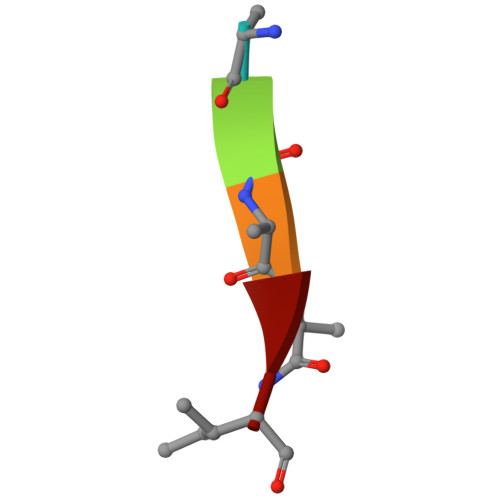> CYYKI> SNATEELTTVRDACARTLENTARTLHLGASGTEFVAAFRAMTDHWGAARPHDLPLSDVSPDGSPVEYAVDLGGLAPALQFAMEPLTAGVPARDPLAARAIMPLLAGRYGADATRWSALADRLLPDDAHGPHVSMYGAEVRA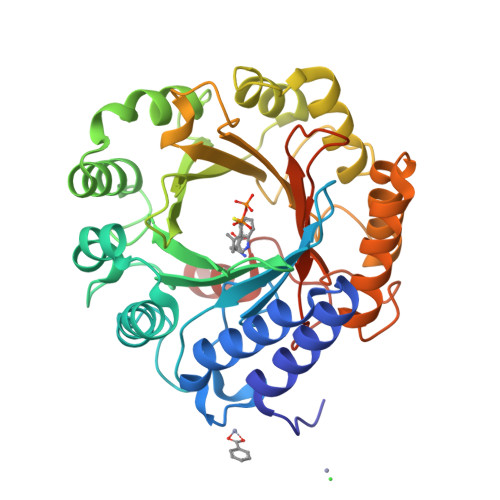GAPIRFKAWFYLNVTGPDGAFNLLYSALERMGTTHLWPVVQAHVHRAGEDVPFLLSLDLSDDPAARVKVYFRHFAADVEEVAAVLKAYPGFEPGEVRAFCKVMMGGRRRFSDQPAVTCVSLLDAQTFDRTAATLYVPLWTYAEHDGEVRQRVHRTLAAWPEALYRYDSVLAGIAHRGLDAGTGIHNYISWQPGRTRPRMKVYLSPEMHDVTPPPLGVSQQHHLSGQTTARGRTE>[2x]STQACPQPKTLDEFTIIQNLQPQYQFRDYFIATCKQGYQLIEGNQVLHSF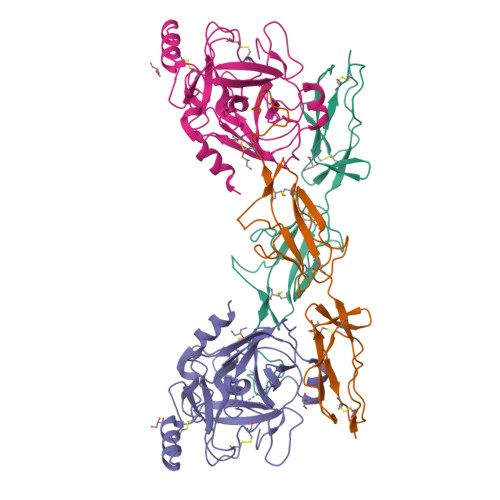TAVCQDDGTWHRAMPRCKIKDCGQPRNLPNGDFRYTTTMGVNTYKARIQYYCHEPYYKMQTRAGSRESEQGVYTCTAQGIWKNEQKGEKIPRCLPVCGKPVNPVEQRQR;>IIGGQKAKMGNFPWQVFTNIHGRGGGALLGDRWILTAAHTLYPKEHEAQSNASLDVFLGHTNVEELMKLGNHPIRRVSVHPDYRQDESYNFEGDIALLELENSVTLGPNLLPICLPDNDTFYDLGLMGYVSGFGVMEEKIAHDLRFVRLPVANPQACENWLRGKNRMDVFSQNMFCAGHPSLKQDACQGDSGGVFAVRDPNTDRWVATGIVSWGIGCSRGYGFYTKVLNYVDWIKKEMEEED[2x]>[2x]G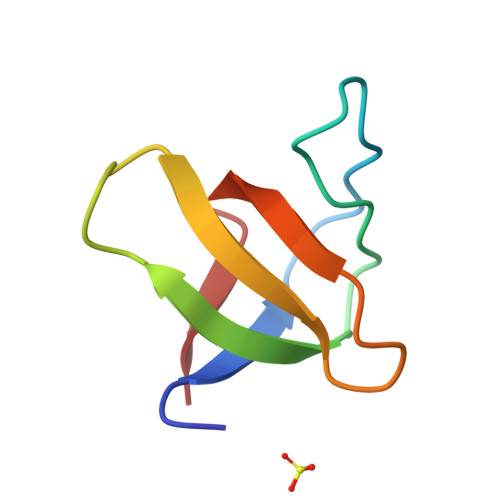MERGIVQYDFMAESQDELTIKSGDKVYILDDKKSKDWWMCQLVDSGKSGLVPAQFIEPV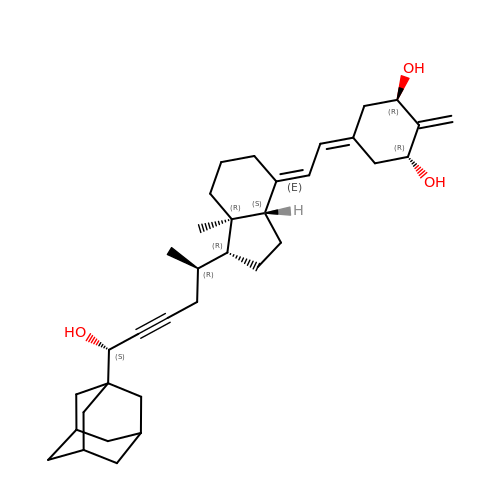(1R,3R,7E,17beta)-17-{(2R,6S)-6-hydroxy-6-[(3S,5S,7S)-tricyclo[3.3.1.1~3,7~]dec-1-yl]hex-4-yn-2-yl}-2-methylidene-9,10-secoestra-5,7-diene-1,3-diol | C35 H50 O3 | RDOXAQMJPJCGHT-KJUWVWBVSA-N>EKQLMNVEPIHADILLETYKRKIADEGRPFLAEFQSIPRVFSKFPIKEARKPFNQNKNRYVDILPYDYNRVELSEINGDAGSNYINASYIDGFKEPRKYIAAQGPRDETVDDFWRMIWEQKATVIVMVTRCEEGNRNKCAEYWPSMEEGTRAFGDVVVKINQHKRCPDYIIQKLNIVNKKEKATGREVTHIQFTSWPDHGVPEDPHLLLKLRRRVNAFSNFFSGPIVVHSSAGVGRTGTYIGIDAMLEGLEAENKVDVYGYVVKLRRQRCLMVQVEAQYILIHQALVEYNQFGETEVNLSELHPYLHNMKKRDPPSEPSPLEAEFQRLPSYRSWRTQHIGNQEENKSKNRNSNVIPYDYNRVPLKHELEMSKESEHDSDESSDDDSDSEEPSKYINASFIMSYWKPEVMIAAQGPLKETIGDFWQMIFQRKVKVIVMLTELKHGDQEICAQYWGEGKQTYGDIEVDLKDTDKSSTYTLRVFELRHSKRKDSRTVYQYQYTNWSVEQLPAEPKELISMIQVVKQKLPQKNSSE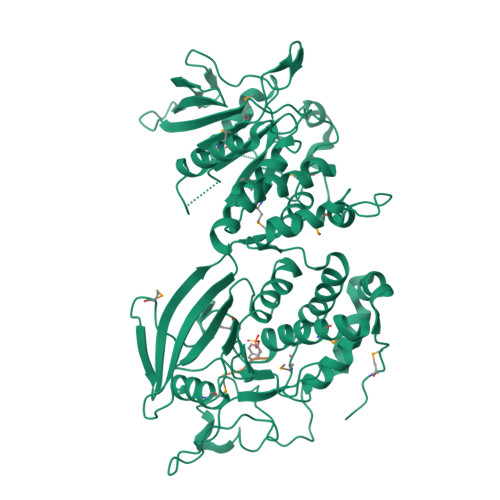GNKHHKSTPLLIHCRDGSQQTGIFCALLNLLESAETEEVVDIFQVVKALRKARLGMVSTFEQYQFLYDVIASTYPAQN[2x];>PTYS[2x]> MSKMDQLRPVLGRAGVDALWVSAPANVRWLSGFTSAEDGKVLVSPDGATLYTDARYTVQAQEESSLPQYIARPPATYEHAADTVRGLRVGFEAESLTVAELEDLRQAWPNSTLVALRGTLGGLRAVKTPEEIGAIRAAQDLADRVYTEVRPMIRAGVRELDVAVEIETRLRRAGGESAFELIVASGPNGAKPHGHASKRVIE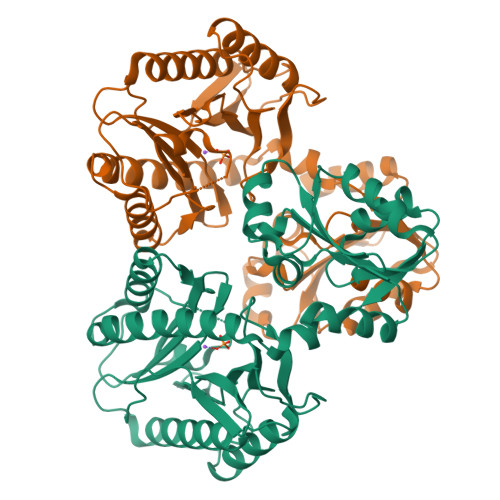DGDLVTIDMGARLGGYNSDMTRTVAVGTPSAEMKRVYDAVLEAEEAAIAAIRPGVRAADLDKLARDLLTRHGLGEAFAHSLGHGVGLEVHEGPGLRGTSQDVLEAGMVITIEPGAYLPGVGGVRIEDLILVTEDGYEVLSHSAKESV> MAKKIITVNVNGKAQEKAVEPRTLLIHFLREELNLTGAHIGCETSHCGACTVDIDGRSVKSCTHLAVQCDGSEVLTVEGLANKGVLHAVQEGFYKEHGLQCGFCTPGMLMRAYRFLQENPNPTEAEIRMGMTGNLCRCTGYQNIVKAVQYAARKLQEP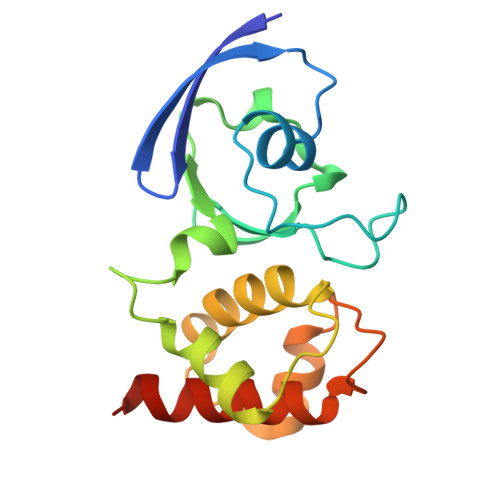STAAA> HMSEPRFVHLHVHSDYSMIDGLAKTAPLVKKAAALGMPALAITDHTNLCGLVKFYGAGHGAGIKPIVGADFNVQCDLLGDELTHLTVLAANNTGYQNLTLLISKAYQRGYGAAGPIIDRDWLIELNEGLILLSGGRMGDVGRSLLRGNSALVDECVAFYEEHFPDRYFLELIRTGRPDEESYLHAAVELAEARGLPVVATNDVHFIDSSDFDAHEIRVAIHDGFTLDDPKRPRNYSPQQYMRSEEEMCELFADIPEALANTVEIAKRCNVTVRLGEYFLPQFPTGDMSTEDYLVKRAKEGLEERLAFLFPDEEERLKRRPEYDERLETELQVINQMGFPGYFLIVMEFIQWSKDNGVPVGPGRGSGAGSLVAYALKITDLDPLEFDLLFERFLNPERVSMPDFDVDFCMEKRDQVIEHVADMYGRDAVSQIITFGTMAAKAVIRDVGRVLGHPYGFVDRISKLIPPDPGMTLAKAFEAEPQLPEIYEADEEVKALIDMARKLEGVTRNAGKHAGGVVIAPTKITDFAPLYCDEEGKHPVTQFDKSDVEYAGLVKFDFLGLRTLTIINWALEMINKRRAKNGEPPLDIAAIPLDDKKSFDMLQRSETTAVFQLESRGMKDLIKRLQPDCFEDMIALVALFRPGPLQSGMVDNFIDRKHGREEISYPDVQWQHESLKPVLEPTYGIILYQEQVMQIAQVLSGYTLGGADMLRRAMGKKKPEEMAKQRSVFAEGAEKNGINAELAMKIFDLVEKFAGYGFNKSHSAAYALVSYQTLWLKAHYPAEFMAAVMTADMDNTEKVVGLVDECWRMGLKILPPDINSGLYHFHVNDDGEIVYGIGAIKGVGEGPIEAIIEARNKGGYFRELFDLCARTDTKKLNRRVLEKLIMSGAFDRLGPHRAALMNSLGDALKAADQHAKAEA

The DNA polymerases at the core of every bacterial replisome belong to the C-family of DNA polymerases. All members of this family contain a set of four domains that are organised within a single polypeptide in the following order: Polymerase and Histidinol Phosphatase (PHP), Palm, Thumb and Fingers. The PHP domain in Pol III and Pol C is a barrel-shaped domain located at the side of the polymerase, near the Thumb domain. In E. coli DNA polymerase III, however, the PHP domain has lost several metal-coordinating residues and is likely to be catalytically inactive.

For this, we made three variants of E. coli Pol III with three, four or five mutations in the PHP domain, termed 3mPHP, 4mPHP, and 5mPHP, respectively. The first of these mutants, 3mPHP, has three histidine residues restored at positions 1, 4 and 9 (i.e. R10H, F44H, R203H). We crystallized 3mPHP under similar conditions to the wild-type protein, and the structure was determined by molecular replacement and refined to 2.9 Å resolution. The 3mPHP structure is virtually identical to that of the wild-type protein, with a root square mean deviation of 0.92 Å over 756 aligned Cα atoms. Two strong peaks (5.0 σ and 6.1 σ) that stand out in the anomalous difference map calculated using X-rays of 1.000 Å wavelength, indicate the presence of two metals bound to the active site of the PHP domain, even though no metals were added to the crystallisation conditions. The positions of the two metal ions in the 3mPHP structure are essentially identical to the metal positions in other PHP domain structures, including T. aquaticus Pol III. A third metal ion often found in canonical PHP domains is not observed. The two metal ions in the 3mPHP structure were, therefore, modelled as zinc. In contrast, wild-type E. coli Pol III shows only a very low level of exonuclease activity. Likewise, the mutants 3mPHP and 4mPHP do not show increased 3′-5′ exonuclease activity relatively to the wild-type protein in the presence of any of the metals tested (Zn2+, Ni2+, Mn2+, Co2+, Cu2+; Figure 5 and data not shown), which may be explained by the fact that these mutants do not have all 5 missing residues restored. Here too, we find that the protein apparently unfolds in a single step, with the 3mPHP mutant being less stable than the wild-type protein.> MGIINIQDEINNYMKEVYGATTVKSTYDPSFKVFNESVTPQFTEIPTEPVNNQLTTKRVDNTGSYPVESTVSFTWTETHTE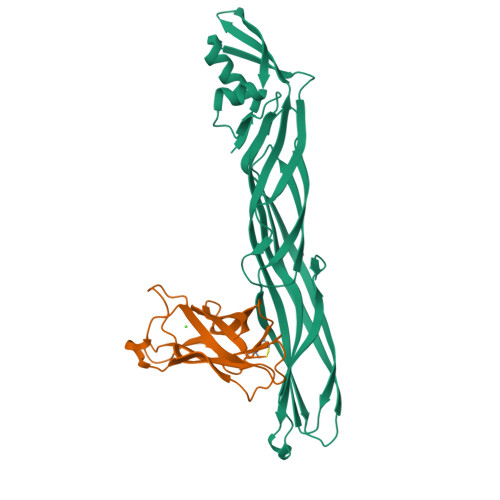TSAVTEGVKAGTSISTKQSFKFGFVNSDVTLTVSAEYNYSTTNTTTTTETHTWSDSTKVTIPPKTYVEAAYIIQNGTYNVPVNVECDMSGTLFCRGYRDGALIAAVYVSVADLADYNPNLNLTNKGDGIAHFKGSGFIEGAQGLRSIIQVTEYPLDDNKGRSTPITYLINGSLAPNVTLKNSNIKF;> MTVYNATFTINFYNEGEWGGPEPYGYIKAYLTNPDHDFEIWKQDDWGKSTPERSTYTQTIKISSDTGSPINQMCFYGDVKEYDVGNADDILAYPSQKVCSTPGVTVRLDGDEKGSYVTIKYSLTPA> MDRRFYGKIVIKGKIKAVTGLHIGSQRDISEIGGIDNPVIKDPHTGLPYIPGSSLKGRLRSLFEILVNSRLGEWREKYPSLANYSPGSCRPDNQENCGKFFNRKINRGWIHVCPDYETALACPVCRLFGASGKESNFPSRIIVRDAFLTKEWEEKWRAGEAITEAKIEVGIDRVTSQANPRTNERVVAGAEFEFEIIYNVENTTHWRDDIKNLLTAMALLEDSYLGGSGSRGYGKVKFIF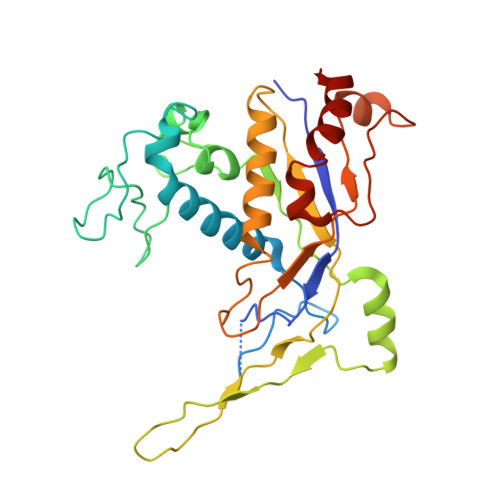DSFEFRPLDYYRTGKDEDIVSIDAREKSVSDILSGFDSLFSEVEGKLEAG>MEGPAGYLRRASVAQLTQELGTAFFQQQQLPAAMADTFLEHLCLLDIDSEPVAARSTSIIATIGPASRSVERLKEMIKAGMNIARLNFSHGSHEYHAESIANVREAVESFAGSPLSYRPVAIALDTKGPEIRTGILQGGPESEVELVKGSQVLVTVDPAFRTRGNANTVWVDYPNIVRVVPVGGRIYIDDGLISLVVQKIGPEGLVTQVENGGVLGSRKGVNLPGAQVDLPGLSEQDVRDLRFGVEHGVDIVFASFVRKASDVAAVRAALGPEGHGIKIISKIENHEGVKRFDEILEVSDGIMVARGDLGIEIPAEKVFLAQKMMIGRCNLAGKPVVCATQMLESMITKPRPTRAETSDVANAVLDGADCIMLSGETAKGNFPVEAVKMQHAIAREAEAAVYHRQLFEELRRAAPLSRDPTEVTAIGAVEAAFKCCAAAIIVLTTTGRSAQLLSRYRPRAAVIAVTRSAQAARQVHLCRGVFPLLYREPPEAIWADDVDRRVQFGIESGKLRGF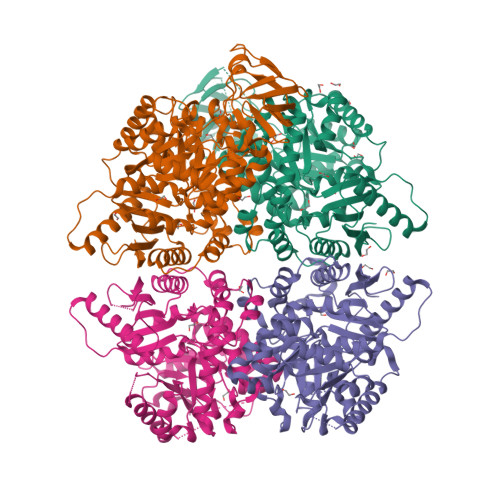LRVGDLVIVVTGWRPGEGYTNIMRVLSIS[8x]>[41x]MALTVNTNIASLNTQRNLNASSNDLNTSLQRLTTGYRINSAKDDAAGLQISNRLSNQISGLN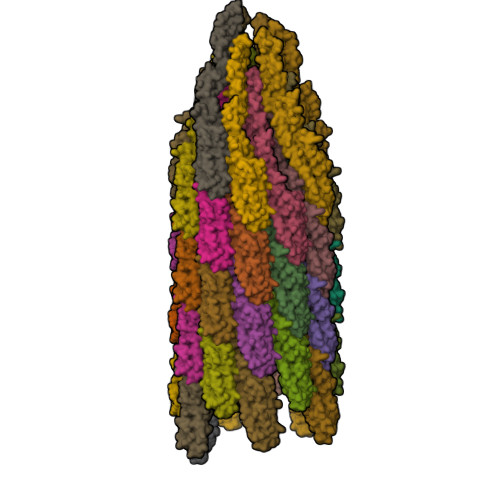VATRNANDGISLAQTAEGALQQSTNILQRIRDLALQSANGSNSDADRAALQKEVAAQQAELTRISDTTTFGGRKLLDGSFGTTSFQVGSNAYETIDISLQNASASAIGSYQVGSNGAGTVASVAGTATASGIASGTVNLVGGGQVKNIAIAAGDSAKAIAEKMDGAIPNLSARARTVFTADVSGVTGGSLNFDVTVGSNTVSLAGVTSTQDLADQLNSNSSKLGITASINDKGVLTITSATGENVKFGAQTGTATAGQVAVKVQGSDGKFEAAAKNVVAAGTAATTTIVTGYVQLNSPTAYSVSGTGTQASQVFGNASAAQKSSVASVDISTADGAQNAIAVVDNALAAIDAQRADLAAVQNRFKNTIDNLTNISENATNARSRIKDTDFAAETAALSKNQVLQQAGTAILAQANQLPQAVLSLLR>ILDTKPIPTIVDATTLGISGNTSGDYWLPTTMSLYQKELTDQIVSLHYSDILRYFETSHYKEDVILESMKTMCLNGSLVATHPYLLIDHYMPKSLITRDVPAHLAENSGKFSVLRDLINLVQEYETETAIVCRPGRTMDLLEALLLGNKVHIKRYDGHSIKSAAAANDFSCTVHLFSSEGINFTKYPIKSKARFDMLICLDTTVDTSQKDIQYLLQYKRERKGLERYAPIVRLVAINSIDHCRLFFGKKFDKNSREYLENVTAAMVILRD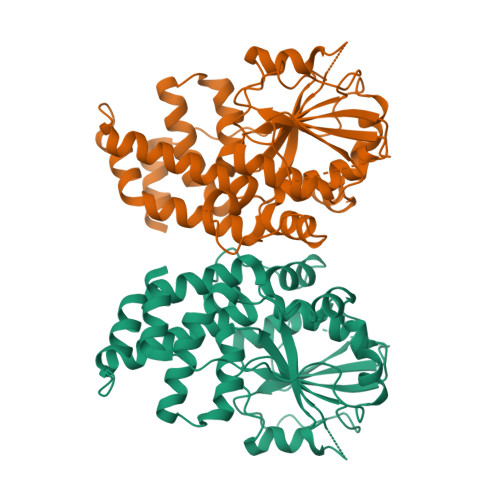RLGTLPPDLRPIYSQKLHYLVEWLENPTVPWPLPDIYPLKQYTSMDVERSLLTEVHFK[2x]>MAHHHHHHVDDDDKENLYFQSKPYISAKDLKEIMYDHLPGFGTAFHQLVQVICKIGKDNNLLDTIHAEFQASLA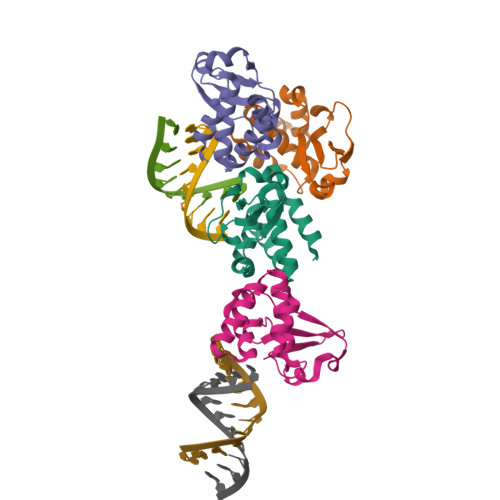DGDSPQCALIQITKRVPIFQDVPPPIIHIRSRGDIPRACQKSLRPAPPSPKIDRGWVCLFKMQDGKTLGLKI[4x]> MRPTFPALGSRAKGYENRVMVYAHRRHRAWYLPPKLAHARSPLANKSPDEYGNTWDPRTGVEWYHRLRRRGAYRHWPWARWNDDPVRQHQELSCRRTFSAAVTGANEGVPL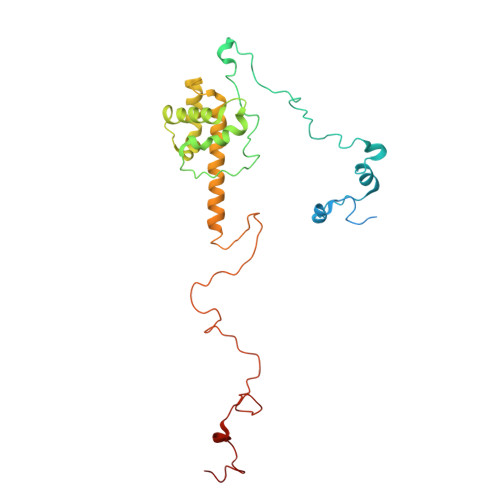WNYYAEVGQEYGLPSHFPLSFMAPFIHQYTSRAWSRKEIERHLKVVEERTGLRTIQQACDATSELLEWGEEEMGVVPHGLLQHVVMLAEDIVLQNKKKAYRKAAHERGILRTTTMERYYALPHLRTGPPMPTTLEQPSGEFPWGKFSTMVGGTRIHPLYRPDGFFKDNMYPA>GQIQISKHVKDVGLPSIHTPTKTKLQPSVFYDIFPGSKEPAVLTEKDPRLKVDFDSALFSKYKGNTECSLNEHIQVAVAHYSAQLATLDIDPQPIAMEDSVFGMDGLEALDLNTSAGYPYVTLGIKKKDLINNKTKDISKLKLALDKYGVDLPMITFLKDELRKKDKIAAGKTRVIEASSINDTILFRTVYGNLFSKFHLNPGVVTGCAVGCDPETFWSKIPLMLDGDCIMAFDYTNYDGSIHPIWFKALGMVLDNLSFNPTLINRLCNSKHIFKSTYYEVEGGVPSGCSGTSIFNSMINNIIIRTLVLDAYKHIDLDKLKIIAYGDDVIFSYKYKLDMEAIAKEGQKYGLTITPADKSSEFKELDYGNVTFLKRGFRQDDKYKFLIHPTFPVEE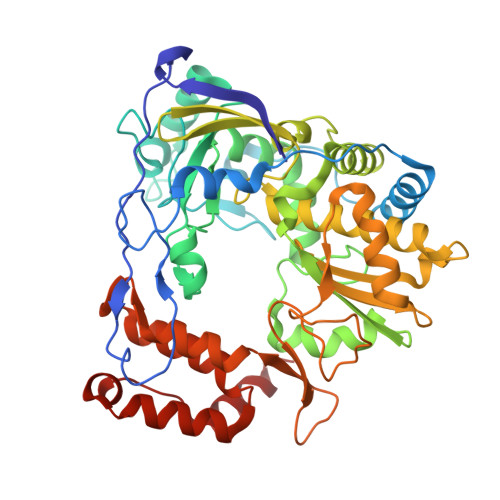IYESIRWTKKPSQMQEHVLSLCHLMWHNGPEIYKDFETKIRSVSAGRALYIPPYELLRHEWYEKF[2x]>[4x]MTMAKLTESMTNVLEGDSMDQDVESPVAIHQPKLPKQARDDLPRHISRDRTKRKIQRYVRKDGKCNVHHGNVRETYRYLTDIFTTLVDLKWFFNLLIFVMVYTVTWLFFGMIWWLIAYIRGDMDHIEDPSWTPCVTNLNGFVSAFLFSIETETTIGYGYRVITDKCPEGIILLLIQSV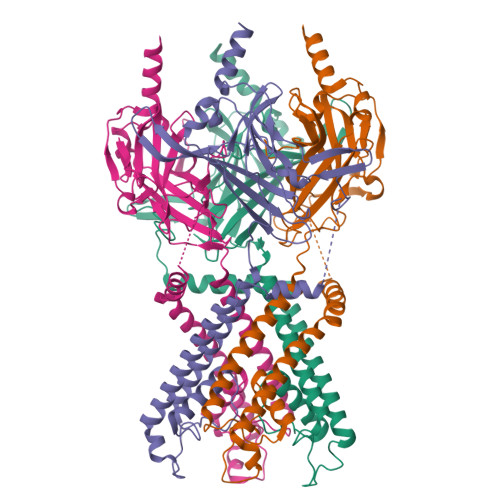LGSIVNAFMVGCMFVKISQPKKRAETLVFSTHAVISMRDGKLCLMFRVGDLRNSHIVEASIRAKLIKSKQTSEGEFIPLNQTDINVGYYTGDDRLFLVSPLIISHEINQQSPFWEISKAQLPKEELEIVVILEGMVEATGMTCQARSSYITSEILWGYRFTPVLTLEDGFYEVDYNSFHETYETSTPSLSAKELAELANRAESPLSWSVSSKLNQHAELETEEEEKNPEELTERNGDVANLENESKS> TKGKATVAFAREARTEVRKVIWP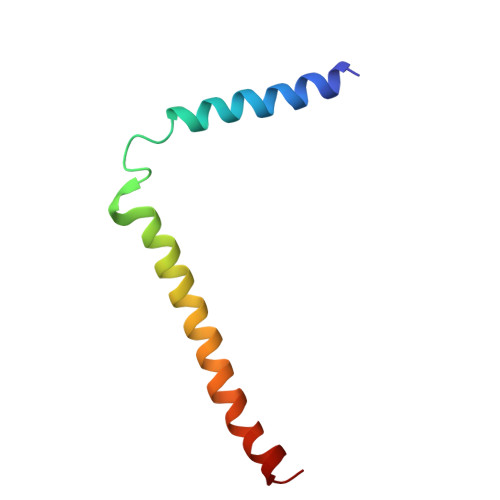TRKPTKDEYLAVAKVTALGISLLGIIGYIIHVPATYIKGILK>[2x]APRKFFVGGNWKMNGDKKSLGELIHTLNGAKLSADTEVVCGAPSIYLDFARQKLDAK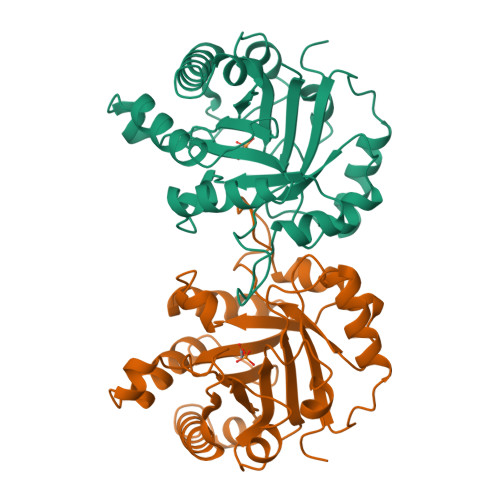IGVAAQNCYKVPKGAFTGEISPAMIKDIGAAWVILGHSERRHVFGESDELIGQKVAHALAEGLGVIACIGEKLDEREAGITEKVVFEQTKAIADNVKDWSKVVLAYDPVWAIGTGKTATPQQAQEVHEKLRGWLKTHVSDAVAQSTRIIYGGSVTGGNCKELASQHDVDGFLVGGASLKPEFVDIINAKH(2S)-3-{4-[2-(4-{[(2R)-2-hydroxy-3,3-dimethylbutyl]oxy}phenyl)propan-2-yl]phenoxy}propane-1,2-diol 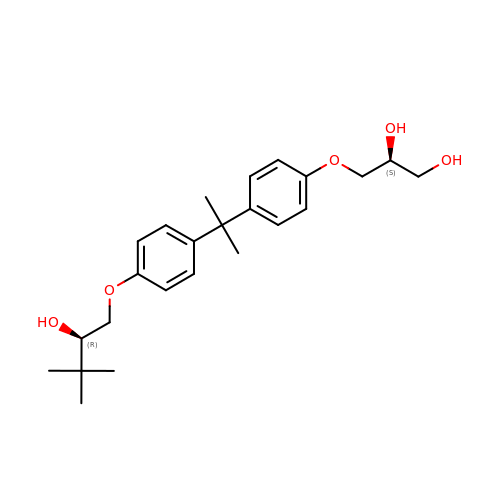| C24 H34 O5 | NSXHQTLHHLJUGK-UGKGYDQZSA-N> MHHHHHHHHRGVRRILPFLGPAVIASIAYMDPGNFATNIEGGARYGYSLLWVILAANLMAMVIQNLSANLGIASGRNLPELIRERWPRPLVWFYWIQAELVAMATDLAEFLGAALAIQLLTGLPMFWGAVVTGVVTFWLLNLQKRGTRPLELAVGAFVLMIGVAYLVQVVLARPDLAAVGAGFVPRLQGPGSAYLAVWIIGATVMPHVIYLHSALTQGRIQTDTTEEKRRLVRLNRVDVIAAMGLAGLINMSMLAVAAATFHGKNVENAGDLTTAYQTLTPLLGPAASVLFAVALLASGLSSSAVGTMAGDVIMQGFMGFHIPLWLRRLITMLPAFIVILLGMDPSSVLILSQVILCFGVPFALVPLLLFTARRDVMGALVTRRSFTVIGWVIAVIIIALNGYLLWELLGG

Transporters of the Nramp (Natural resistance-associated macrophage protein) family import divalent transition metal ions into cells of most organisms. In addition to the physiological substrates Fe2+ and Mn2+, Nramps can also transport toxic metals like Cd2+ and Hg2+ but exclude the abundant alkaline earth metals like Mg2+ and Ca2+. Recent bacterial Nramp structures reveal a LeuT fold, three stable conformations (outward-open, occluded, and inward-open), and identify the metal-binding site residues, including conserved aspartate, asparagine, and methionine residues. We present high-resolution structures of DraNramp in three conformations in both Mn2+-bound and metal-free states, providing the first molecular map of the entire Mn2+ transport cycle.

We also determined high-resolution DraNramp structures in metal-free occluded (WT) and Mn2+-bound inward-open (M230A•Mn2+) states and re-refined a Mn2+-bound outward-open conformation (G223W•Mn2+). Re-refined G223W•Mn2+ has six Mn2+-coordinating ligands: D56, N59, M230, carbonyl of A53 and two waters; the overall geometry resembles a distorted octahedron as in the occluded structure. A227 replaces a water of the outward-open Mn2+-coordination sphere, thus retaining a six-coordination geometry in both conformations. In the occluded and inward-open conformations, Q378 interacts with two waters, one coordinating the orthosteric Mn2+ and the other interacting with D56 and the carbonyl of T130. This network is disrupted in the outward-open conformation as Q378 and the rest of TM10 swing outward to open the outer vestibule. In the second network, T228, N275, and N82 interact via a water in the occluded and inward-open states, but not in the outward-open state, where the extended unwound region of TM6a positions T228 farther from the orthosteric site and N275 and N82. In the outward-open state, R244 forms an ion pair with E176 and interacts with the TM1a backbone, as does D263, keeping TM1a and TM5 close and the inner gate closed (Bozzi et al., 2020). A metal ion is present at the external site in all inward-open and occluded metal-bound DraNramp structures, but not outward-open structures, as opening the outer vestibule separates D296 and D369 and disrupts the site. The ITC data for G223W with Mn2+ fits only in a one-site model (Kd=440±15 µM), which we assign to the orthosteric site because the opening of the outer vestibule displaces TM10, disrupting the external site. Mn2+ binds at the orthosteric site in G223W, but Cd2+ binding is impaired.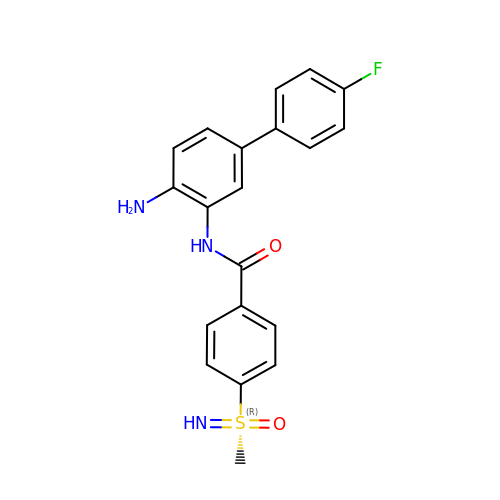(R)-N-(4-amino-4'-fluoro-[1,1'-biphenyl]-3-yl)-4-(S-methylsulfonimidoyl)benzamide | C20 H18 F N3 O2 S | JPFMYSJUFUEHBI-HHHXNRCGSA-N>[2x]MDDGGELSLVKKVVHSLVV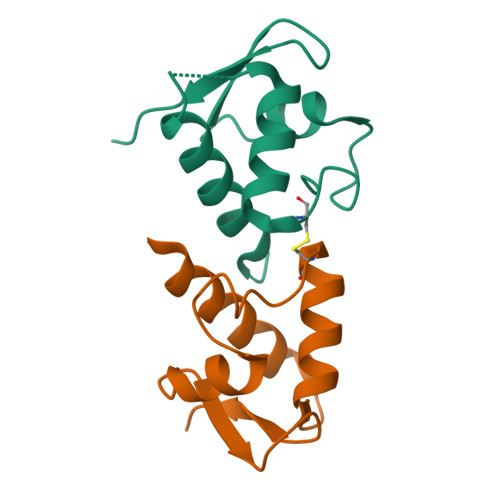SSPGKLTVEQLMRDYRSAAGCTLPYSKLGFKDAESFLRSIPDTVTVTGHGQMAWITAVATA> MCPPGWSSNGVYCYMLFKEPKTWDEAEKFCNKQGKDGHLLSIESKKEEILVDIVVSENIGK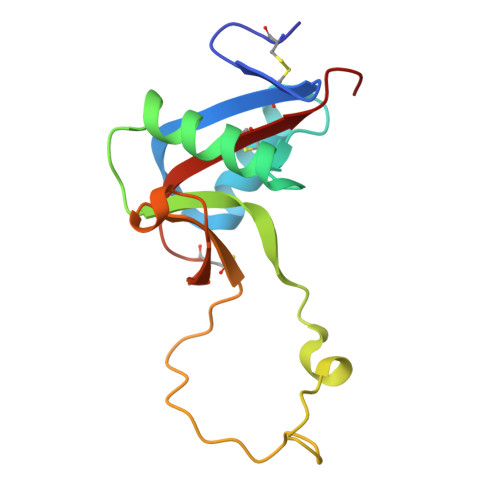MYKIWTGLSERSKEQHCSSRWSDGSFFRSYEIAIRYSECFVLEKQSVFRTWVATPCENTFPFMCKYPVPR> MGSINLRIDDELKARSYAALEKMGVTPSEALRLMLEYIADNERLPFKQTLLSDEDAELVEIVKERLRN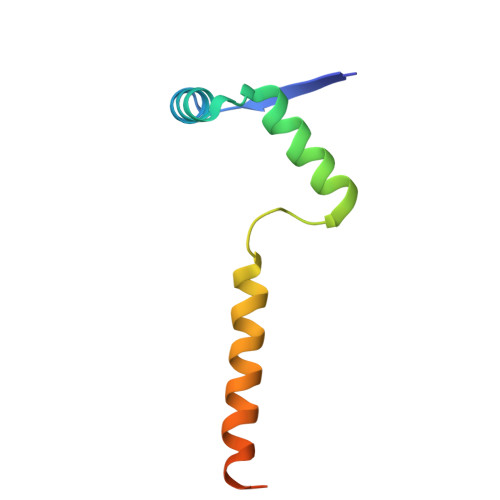PKPVRVTLDEL> MKIFSESHKTVFVVDHCPYMAESCRQHVEFDMLVKNRTQGIIPLAPISKSLWTCSVESSMEYCRIMYDIFPFKKLVNFIVSDSGAHVLNSWTQEDQNLQELMAALAAVGPPNPRADPECCSILHGLVAAVETLCKITEYQHEARTLLMENAERVGNRGRIICITNAKSDSHVRMLEDCVQETIHEHNKLAANSDHLMQIQKCELVLIHTYPVGEDSLVSDRSKKELSPVLTSEVHSVRAGRHLATKLNILVQQHFDLASTTITNIPMKEEQHANTSANYDVELLHHKDAHVDFLKSGDSHLGGGSREGSFKETITLKWCTPRTNNIELHYCTGAYRISPVDVNSRPSSCLTNFLLNGRSVLLEQPRKSGSK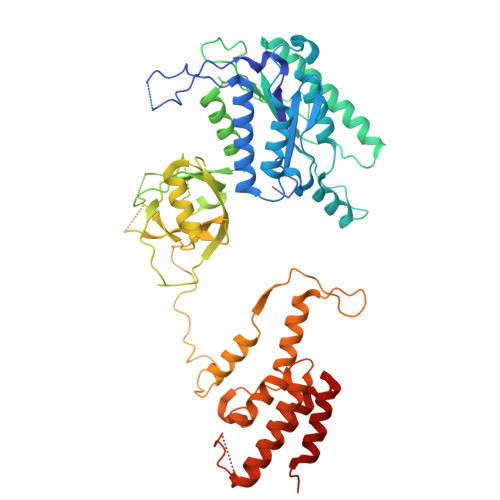VISHMLSSHGGEIFLHVLSSSRSILEDPPSISEGCGGRVTDYRITDFGEFMRENRLTPFLDPRYKIDGSLEVPLERAKDQLEKHTRYWPMIISQTTIFNMQAVVPLASVIVKESLTEEDVLNCQKTIYNLVDMERKNDPLPISTVGTRGKGPKRDEQYRIMWNELETLVRAHINNSEKHQRVLECLMACRSKP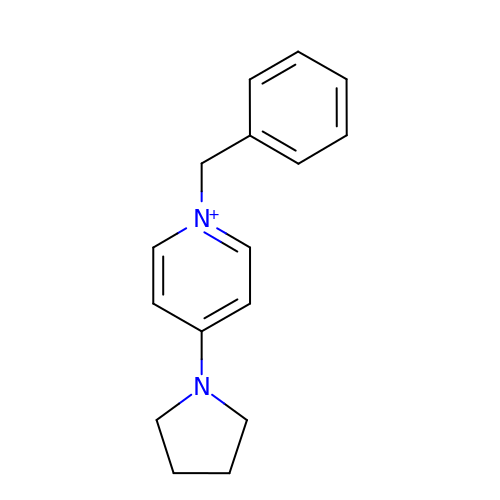1-(phenylmethyl)-4-pyrrolidin-1-yl-pyridin-1-ium | C16 H19 N2 | HEIRUXZPJJZCAO-UHFFFAOYSA-N The classical inhibitors of DHFR have reduced activity against Leishmania and Trypanosoma due to the upregulation of a gene encoding the dihydronicotinamide adenine dinucleotide phosphate (NADPH)-dependent pteridine reductase 1 (PTR1). PTR1 is present in Leishmania spp. and Trypanosoma brucei parasites, but not in the human cells. It is able to reduce both unconjugated and conjugated pterins and provides a metabolic bypass to alleviate DHFR inhibition. PTR1 is a functional homotetramer with four catalytic sites. Each subunit has a single α/β structured domain with the typical topology of short-chain dehydrogenases/reductases (SDR) and is characterized by a seven-stranded parallel β-sheet sandwiched by three α-helices on each side, that represents the classical dinucleotide-binding motif known as the Rossmann fold.

Moreover, these experiments provided the first X-ray crystallographic structures of LmPTR1 in complex with chroman-4-one derivatives (compounds 1 and 3). The orientations of compounds 1 and 3 in the catalytic pocket of LmPTR1 resemble that of compound 1 in the TbPTR1 active site. The chroman-4-one scaffold establishes a π-sandwich between the nicotinamide of NADP+ and Phe113 and most of the interactions with the surrounding residues are retained across the two species: the hydroxyl group in position 6 of both compounds is located within H-bonding distance of the β-phosphate oxygen atom O2A of NADP+, and Ser111 side chain. In both compounds, the carbonyl group in position 4 is H-bonded to the NH2 group of Arg17. As in TbPTR1, the phenol moieties are located in a prevalently hydrophobic pocket lined by Leu188, Leu226, Leu229, His241 and Arg287 (for clarity, leucine residues are not labelled in Figure 3B–D). In the complex LmPTR1-3, the involvement of the m-hydroxyl group of the catechol ring in the interaction with the NH2 group of Arg287 is visible only in chains C and D, whereas in chains A and B, due to a flip of the catechol ring of about 120°, the p-hydroxyl group interacts with the side chain of Tyr283. On the other hand, the crystal structure of LmPTR1 with compound 3 reveals a binding mode different from that of compound 1. For example, His241 lies at about 4 Å from ring B of 3 and is part of an alpha-helix adjacent to the substrate loop. Irrespective of the compound in the catalytic pocket, different conformations of His241 in LmPTR1, at the corresponding position of Trp221 of TbPTR1, were observed in the tetramer, indicating a high flexibility of this residue which delimits the catalytic pocket. All three flavanones show a percentage of inhibition of LmPTR1 greater than 50%, with compounds 2 and 3 being the most active (IC50 35 and 36 µM, respectively).

>MTAPTVPVALVTGAAKRLGRSIAEGLHAEGYAVCLHYHRSAAEANALSATLNARRPNSAITVQADLSNVATAPVSGADGSAPVTLFTRCAELVAACYTHWGRCDVLVNNASSFYPTPLLRNDEDGHEPCVGDREAMETATADLFGSNAIAPYFLIKAFAHRVAGTPAKHRGTNYSIINMVDAMTNQPLLGYTIYTMAKGALEGLTRSAALELAPLQIRVNGVGPGLSVLVDDMPPAVWEGHRSKVPLYQRDSSAAEVSDVVIFLCSSKAKYITGTCVKVDGGYSLTRA[4x]> ADVILFPSK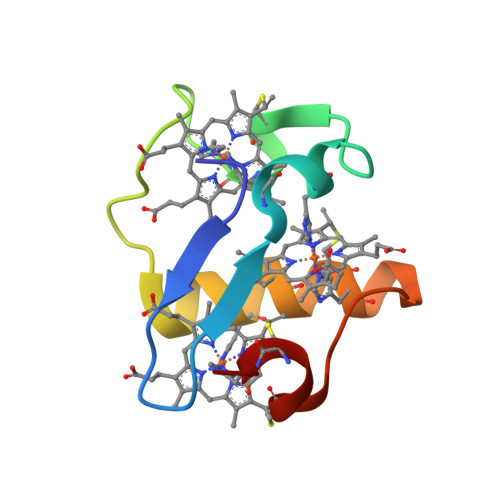NGAVTFTHKRHSEFVRECRSCHEKTPGKIRNFGKDYAHKTCKGCHEVRGAGPTKCKLCHTG> MTDNTRLRIAMQKSGRLSDDSRELLARCGIKINLHTQRLIAMAENMPIDILRVRDDDIPGLVMDGVVDLGIIGENVLEEELLNRRAQGEDPRYFTLRRLDFGGCRLSLATPVDEAWDGPLSLNGKRIATSYPHLLKRYLDQKGISFKSCLLNGSVEVAPRAGLADAICDLVSTGATLEANGLREVEVIYRSKACLIQRDGEMEESKQQLIDKLLTRIQGVIQARESKYIMMHAPTERLDEVIALLPGAERPTILPLAGDQQRVAMHMVSSETLFWETMEKLKALGASSILVLPIE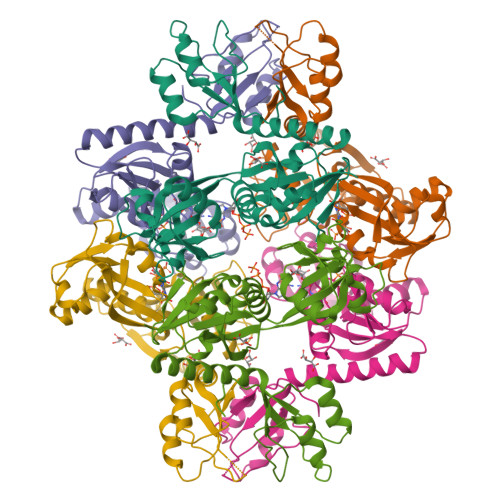KMME> MITDCFEADIAIPSGISRPDAAALQRCEGRVVFLPTIRRQLALADVAHESFVSGGVSPDTLGLLLAYRRRFPAVITRVLPTRIVACPVDLGLTHAGTVNLRNTSPVDLCNGDPVSLVPPVFEGQATDVRLESLDLTLRFPVPLPTPLAREIVARLVARGIRDL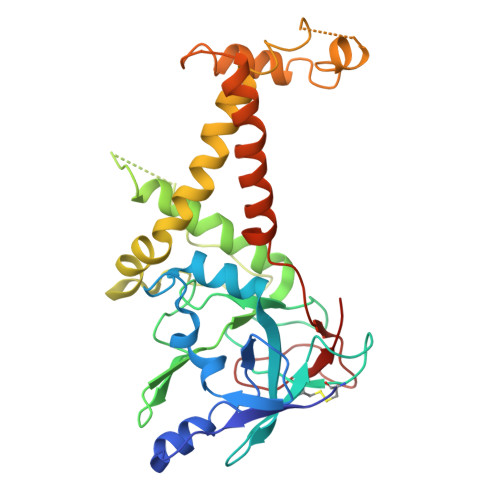NPDPRTPGELPDLNVLYYNGARLSLVADVQQLASVNTELRSLVLNMVYSITEGTTLILTLIPRLLALSAQDGYVNALLQMQSVTREAAQLIHPEAPMLMQDGERRLPLYEALVAWLAHAGQLGDILALAPAVRVCTFDGAAVVQSGDMAPVIRYP>[2x]SMLWVGVVSIFPEMFRAISDYGITSRAVKQGLLTLTCWNPRVYTEDRHQTVDDRPFGGGPGMVMKIKPLEGALADARQAA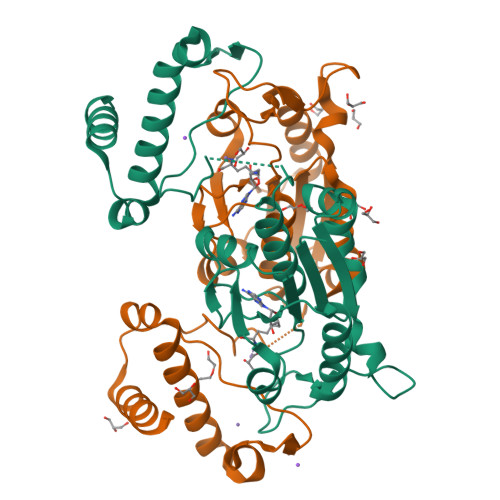GGRKAKVIYLSPQGRQLTQAGVRELAEEEALILIAGRYEGIDERFIEEHVDEEWSIGDYVLSGGELPAMVLVDAVTRLLPGALGHADSAEEDSFTDGLLDCPHYTRPEVYADKRVPEVLLSGNHEHIRRWRLQQALGRTWERRADLLDSRSLSGEEQKLLAEYIRQRDDS> MEIDFEDDIDFDVYFRKTK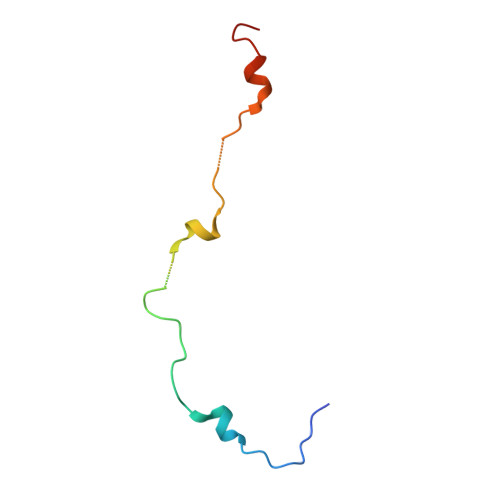AATILTKSTLENQNWRATTLPTDFNYNVDTLVQLHLKP>[2x]SFKDLNLTDAQKQQIREIMKGQRDQMKRPPLEERRAMHDIIASDTFDKVKAEAQIAKMEEQRKANMLALMETQNKIYNILTPEQKKQFNANFEKRLT

Spy is one of a group of chaperones that allow clients to fold while remaining continuously bound to the surface of the chaperone. We have previously observed that the chaperone substrate Im7 exists in a heterogeneous, largely disordered crystallographic ensemble while bound to the chaperone Spy. To refine strategies for detecting anomalous scattering for observing partially occupied disordered states, we co-crystallized the tight-binding Spy H96L variant with short peptides derived from its client, Im7. These peptides each had a single iodophenylalanine substitution at position 18, 19 or 20.

However, other indicators strongly suggest that this ANODE anomalous peak also arises from iodine. (i) The height of the ANODE anomalous peak is the second largest observed in this study and, at 26.4σ in the phased anomalous difference Fourier map, is substantially larger than the signals observed from zinc, chlorine and methionine sulfur, the largest of which is 9.3σ. (ii) The position of this anomalous signal is structurally inconsistent with expected zinc- or chlorine-binding residues, which would be required to enable binding with a suffciently high occupancy to produce a strong anomalous signal. Thus, although the 4.5 keV data set was not analyzed for this crystal, the strength of the signal and its chemical environment are inconsistent with it being derived from zinc or chloride, making it likely that the anomalous signal is owing to the iodine in the Im7 peptide. The larger peak heights for L18pI-Phe and K20pI-Phe, compared with each of the L19pI-Phe peaks, suggest a higher level of occupancy at these positions. Attempts to perform traditional model building using the residual L18pI-Phe and K20pI-Phe peptide density were unsuccessful owing to the weak nature of the electron density, as well as its somewhat amorphous shape, which is likely to be owing to multiple conformations within the peptide. Of note, the electron density for the L18pI-Phe and K20pI-Phe mutants has a substantially more defined shape and signal strength than that observed previously in other mutants. In the case of L18pI-Phe, the molecular-dynamics simulation used to generate the conformational pool was found to not sample positions encompassing the iodine position in the crystal, preventing any fitting and further analysis of this signal.> MASVHGTT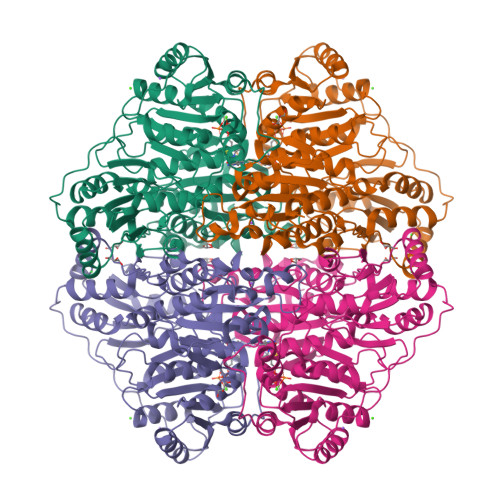YELLRRQGIDTVFGNPGSNELPFLKDFPEDFRYILALQEACVVGIADGYAQASRKPAFINLHSAAGTGNAMGALSNAWNSHSPLIVTAGQQTRAMIGVEALLTNVDAANLPRPLVKWSYEPASAAEVPHAMSRAIHMASMAPQGPVYLSVPYDDWDKDADPQSHHLFDRHVSSSVRLNDQDLDILVKALNSASNPAIVLGPDVDAANANADCVMLAERLKAPVWVAPSAPRCPFPTRHPCFRGLMPAGIAAISQLLEGHDVVLVIGAPVFRYYQYDPGQYLKPGTRLISVTCDPLEAARAPMGDAIVADIGAMASALANLVEESSRQLPTAAPEPAKVDQDAGRLHPETVFDTLNDMAPENAIYLNESPSTTAQMWQRLNMRNPGSYYTCAAGGLGFALPAAIGVQLAEPERQVIAVIGDGSANYSISALWTAAQYNIPTIFVIMNNGTYGILRWFAGVLEAENVPGLDVPGIDFRALAKGYGVQALKADNLEQLKGSLQEALSAKGPVLIEVSTVSPVKRSHHHHHH> ISQFSEAYNKILRNSSSHSSCQLVIFVSCLNIDALCATKMLSLLFKKQLVQSQIVPIFGYSELRRHYSQLDDNINSLLLVGFGGVIDLEAFLEIDPQEYVIDTDEKSGEQSFRRDIYVLDAHRPWNLDNIFGSQIIQCFDDGTVDDTLGEQKEAYYKLLELDEESGDDELSGDENDNNGGDDEATDADEVTDEDEEDEDETISNKRGNSSIGPNDLSKRKQRKKQIHEYEGVLEEYYSQGTTVVNSISAQIYSLLSAIGETNLSNLWLNILGTTSLDIAYAQVYNRLYPLLQDEVKRLTPSSRNSVKTPDTLTLNIQPDYYLFLLRHSSLYDSFYYSNYVNAKLSLWNENGKKRLHKMFARMGIPLSTAQETWLYMDHSIKRELGIIFDKNLDRYGLQDIIRDGFVRTLGYRGSISASEFVEALTALLEVGNSTDKDSVKINNDNNDDTDGEEEEDNSAQKLTNLRKR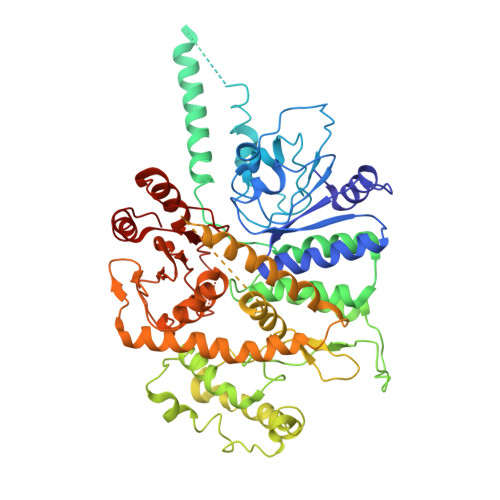WVSNFWLSWDALDDRKVELLNRGIQLAQDLQRAIFNTGVAILEKKLIKHLRIYRLCVLQDGPDLDLYRNPLTLLRLGNWLIECCAESEDKQLLPMVLASIDENTDTYLVAGLTPRYPRGLDTIHTKKPILNNFSMAFQQITAETDAKVRIDNFESSIIEIRREDLSPFLEKLTLSGLL> APVNISKAILLGVILGGLILFGVLGNILVILSVACHRHLHSVTHYYIVNLAVADLLLTSTVLPFSAIFEVLGYWAFGRVFCNIWAAVDVLCCTASIMGLCIISIDRYIGVSYPLRYPTIVTQRRGLMALLCVWALSLVISIGPLFGWRQPAPEDETICQINEEPGYVLFSALGSFYLPLAIILVMYCRVYVVAKRESRGLKSGLKTDKSDSEQVTLRIHRKNAPAGGSGMASAKTKTHFSVRLLKFSREKKAAKTLGIVVGCFVLCWLPFFLVMPIGSFFPDFKPSETVFKIVFWLGYLNS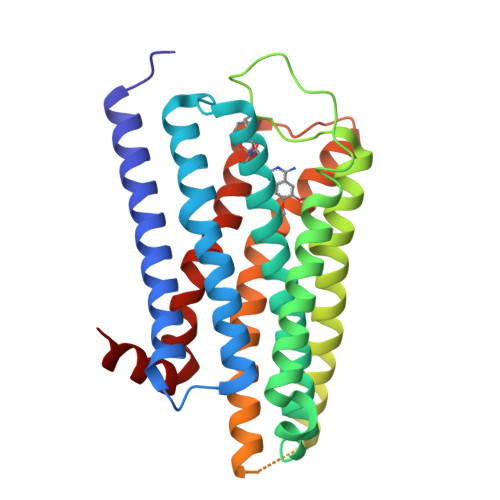CINPIIYPCSSQEFKKAFQNVL> MSAVAGCTATTDPGWEVDA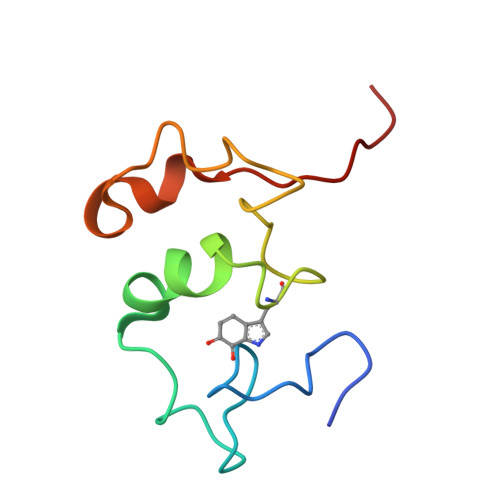FGGVSSLCQPMEADLYGCSDPCWWPAQVPDMMSTYQDWNAQASNSAEDWRNLGTVFPKDK>GSRVAILWHEMWHEGLEEASRLYFGERNVKGMFEVLEPLHAMMERGPQTLKE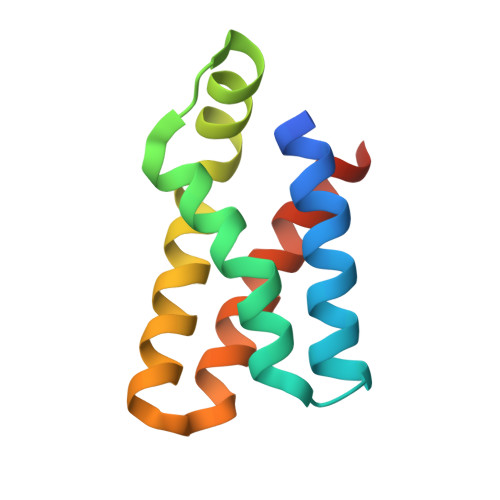TSFNQAYGRDLMEAQEWCRKYMKSGNVKDLTQAWDLYYHVFRRISKQSGG[5x];> TYVAPSVLESVKEKFSFEPKIRSPRR> MGHHHHHHHHHHMRSAVTVLMEHIRNLYLIRRLSLFELKSDNSNQYLGILWEIINPMIQIAIYWFVFGYGIRGRHPVGHIPFILWMLAGMTVWFFVNQAVL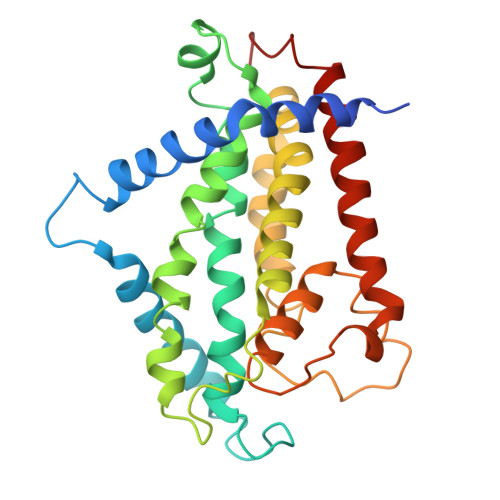QASKSVYTRIRMVAQMNFPISVIPTYVITAKFYQHLMLLAVIFIIFQFTPYHVSVYLVQLPYYMFGLLALLVSFSLITSTLATVVRDVQMIVQSLVRILLYLTPLLWDPSHLPHLVQVIMRLNPLYYIVEGYRSALLGTSWYLVDHASYTVYFWVVVILFFVFGSMVHLKFRAHFVDYM> MEAVPRMPMIWL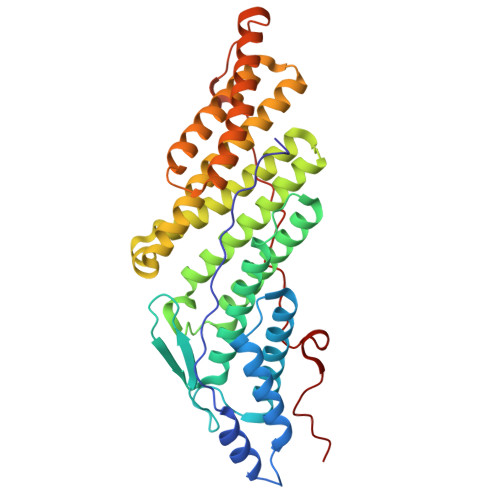DLKEAGDFHFQPAVKKFVLKAAGENPEAYNEELKKLELLRQNAVRVPRDFEGCSVLRKYLGQLHYLQSRVPMGSGQEAAVPVTWTEIFSGKSVAHEDIKYEQACILYNLGALHSMLGAMDKRVSEEGMKVSCTHFQCAAGAFAYLREHFPQAYSVDMSRQILTLNVNLMLGQAQECLLEKSMLDNRKSFLVARISAQVVDYYKEACRALENPDTASLLGRIQKDWKKLVQMKIYYFAAVAHLHMGKQAEEQQKFGERVAYFQSALDKLNEAIKLAKGQPDTVQDALRFTMDVIGGKYNSAKKDNDFIYHEAVPALDTLQPVKGAPLVKPLPVNPTDPAVTGPDIFAKLV> GMLDEYEQAIKRAQENIKKGEELEKKLDKLE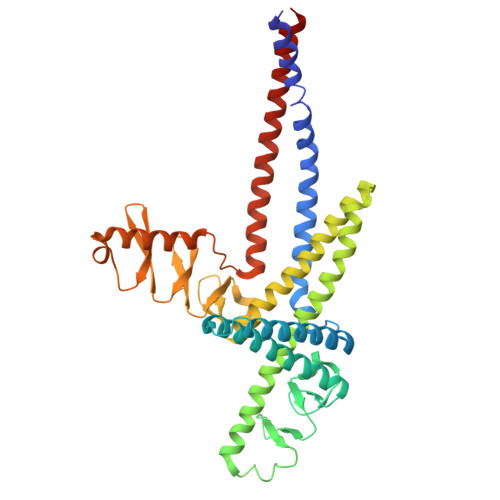RQGKDLEDKYKTYEENLEGFEKLLTDSEELSLSEINEKMEAFSKDSEKLTQLMEKHKGDEKTVQSLQREHHDIKAKLANLQVLHDAHTGKKSYVNEKGNPVSSLKDAHLAINKDQEVVEHEGQFYLLQKGQWDAIKNNPAALEKAQKDYSQSKHDLATIKMEALIHKLSLEMEKQLETINNLIMSTDPKENEEATKLLHKHNGLNLKLANLQDMLAVHRKEKSFFNEKGEEVTSLNDAHYVIGKDQQLFNLGGKFYPIHKEQKILEKDGKFYLLKQGEDWESIKDSPEKQKKAEHDFHKLQYETPMTVKKLVHHNKGLETTIHKERVEETKQQLEDNGKEKIEIANNISKLQS>HGYIAKPAPSWKASKTNNWVVEIEPQWKGGWDESKGDEGLLATFKELAPKNNFKDVRSLMDGNPVFGEECGFTDPKGKPSEPPSDGTATFSRGIVHAGPCEIWLDDKMVLQNDDCQSAYGDGTQQTIAVF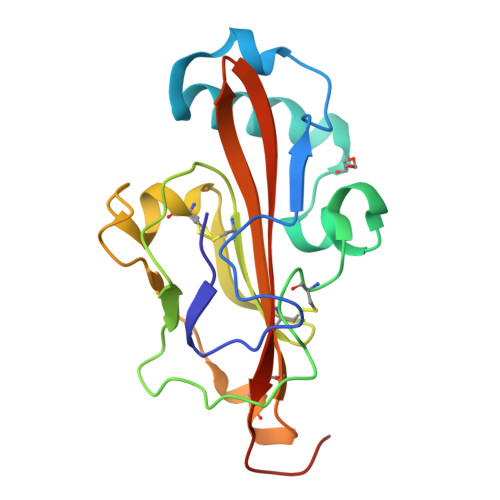KPVDYSSCAAGGCMLRFYWLALQRLKGKTVWQAYKNCIPLTGWSHPQFEK[2x]>[2x]MNHKVHHHHHHIEGRHMITITGYSDVLSAGPGETVEFKVSSKSPHPFTAELVRVIHADPNPAGPGMRFEPLGQVFSGTFASFDKPLLPGSFARVSGVPAAGSAAGLVAGARIRPTALARGDQCV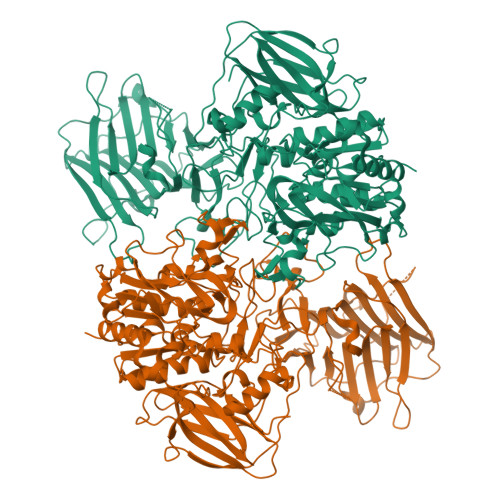MSQWNTARHAGFALLVSERGLELRLGAGTGEPPVCVLCAARLEVRWYDVWFAIDTASNRIEVGVTEVDGSVAAPVRHRTLQMLDARWRAPHSDDAADLLIGALEDGAGRRAHFNGQIEAPFVADALPSPATPAATVEYAAPRASDFSTDALYAAWDFARGIDTLKIADTTPHARHGTLQNLPTRAVRSSAWNGRERCWRTAPAHYAAIHFHDDDLHDAGWSTDFAFTVPATLKSGAYAMRLSVDGATDYLPFYVRPELGRPGAPLVFVAATYTYQAYANYARGNFDAALRDKVGRWGAYPHNPDDHPEVGLATYNLHSDGSGVMFSSRLRPMLTMRPGFLTFDDSRGSGCRHYIADSHLLDWLEHEGFSFDVVTDDDLERFGAALLEPYAAVLTGTHPEYHTAATLDALAGYKRSGGNLAYLGGNGFYWRVGRSERVPGALEVRRTEGGVRAWAAEAGEYFHALDGEYGGLWRSSARTPQQLVGVGFSSQGPFEGSHYRVLDAARSQPGGSLLKDIAGPLFGGYGLSGGGAAGFELDSTEAADGTPANVIILARSESHSAAFGPALDALLSHTATRARKTPDTLIRSEIVYYETGYGGAVFSVGSITFCGALSHNDYRNDVSTLLRNVLIRFSRDRGAQAHAVPAVAHTEVD> GFLVPPTVESRTKPFTVPILTVEEMSNSRFPIPLEKLYTGPSSAFVVQPQNGRCTTDGVLLGTTQLSAVNICTFRGDVTHIAGSHDYIMNLASQNWNNYDPTEEIPAPLGTPDFVGKIQGMLTQTTREDGSTRAHKATVSTGSVHFTPKLGSVQYTTDTNNDLQTGQNTKFTPVGVIQDGNNHQNEPQQWVLPNYSGRTGHNVHLAPAVAPTFPGEQLLFFRSTMPGCSGYPNMNLDCLLPQEWVQHFYQEAAPAQSDVALLRFVNPDTGRVLFECKLHKSGYVTVAHTGPHDLVIPPNGYFRFDSWVNQFYTLAPMGNGAG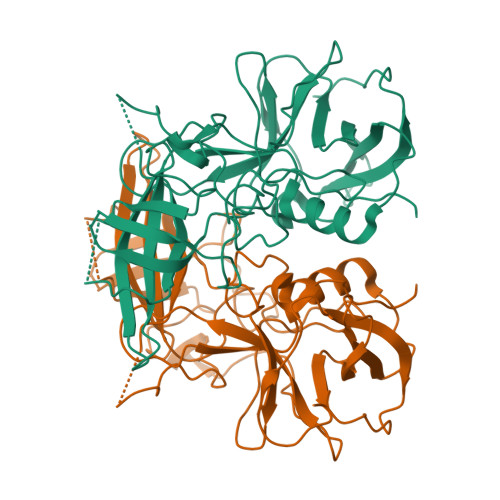RRRAL> RWEQTHLTYRIENYTPDLPRADVDHAIEKAFQLWSNVTPLTFTKVSEGQADIMISFVRGDHR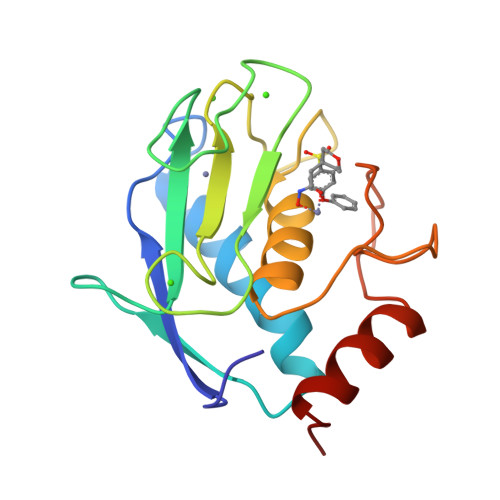DNSPFDGPGGNLAHAFQPGPGIGGDAHFDEDERWTNNFREYNLHRVAAHELGHSLGLSHSTDIGALMYPSYTFSGDVQLAQDDIDGIQAIYGRSQ>PTNRQIVLASRPVGAPTADNFALTQSDIPTPAQGEMLLRSVYLSLDPYMRGRMSDAKSYAEPVGIDEVMVGGTVCQVEASNHAEFEVGEWVLAYTGWQDYALSDGEGLIKLGKQPSHPSYALGVMGMPGFTAYMGLLDIGQPKEGDTLVVAAATGAVGSMVGQIGKLKGCRVIGIAGGEEKCQFAKDTLGFDECIDHKAADFAE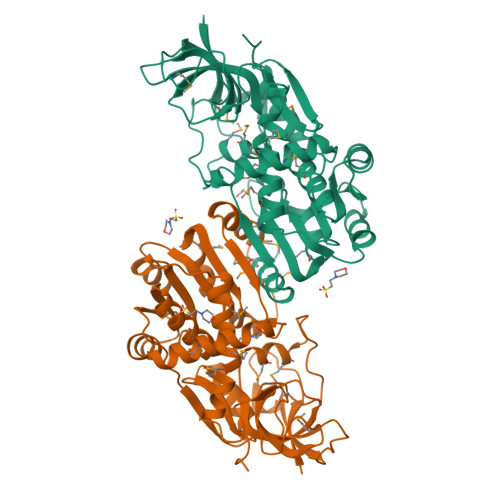QLAKVCHNGIDIYFENVGGKVFDAVMPLLNTGARIPLCGLISQYNATSLPEGPDRMSMLMAQLLIKRIKMQGFIIFDDYGHRYGEFAADMTQWLAQGKIHYREHLVQGLENAPDAFIGLLEGKNFGKMVVQTNQPR[2x]> GSFVEMVDNLRGKSGQGYYVEMTVGSPPQTLNILVDTGSSNFAVGAAPHPFLHRYYQRQLSSTYRDLRKGVYVPYTQGKWEGELGTDLVSIPHGPNVTVRANI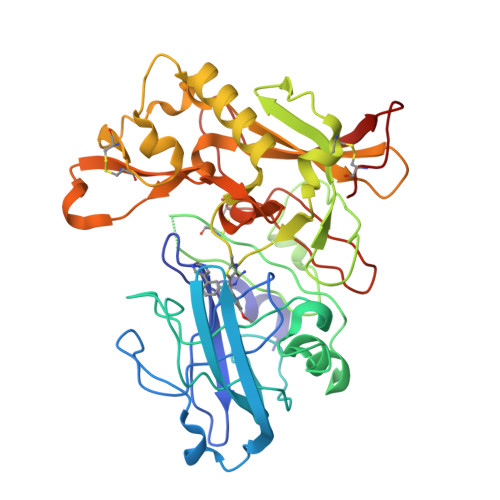AAITESDKFFINGSNWEGILGLAYAEIARPDDSLEPFFDSLVKQTHVPNLFSLQLCGAGFPLNQSEVLASVGGSMIIGGIDHSLYTGSLWYTPIRREWYYEVIIVRVEINGQDLKMDCKEYNYDKSIVDSGTTNLRLPKKVFEAAVKSIKAASSTEKFPDGFWLGEQLVCWQAGTTPWNIFPVISLYLMGEVTNQSFRITILPQQYLRPVEDVATSQDDCYKFAISQSSTGTVMGAVIMEGFYVVFDRARKRIGFAVSACHVHDEFRTAAVEGPFVTLDMEDCGY> GHMERLLDELTLEGVARYMQSERCRRVICLVGAGISTSAGIPDFRSPSTGLYDNLEKYHLPYPEAIFEISYFKKHPEPFFALAKELYPGQFKPTICHYFMRLLKDKGLLLRCYTQNIDTLERIAGLEQEDLVEAHGTFYTSHCVSASCRHEYPLSWMKEKIFSEVTPKCEDCQSLVKPDIVFFGESLPARFFSCMQSDFLKVDLLLVMGTSLQVQPFASLISKAPLSTPRLLINKEKAGQSDPFLGMIMGLGGGMDFDSKKAYRDVAWLGECDQGCLALAELLGWKKELEDLVRREHASIDAQS;> EKR

NAD+-dependent protein deacylases (sirtuins) constitute a unique class of enzymes that are conserved from bacteria to humans. The human isotype Sirtuin 2 (Sirt2) deacetylates both nuclear and cytoplasmatic proteins and thereby functions as a major cell cycle regulator, a determinant of myelination, a regulator of autophagy and a suppressor of brain inflammation. In this work, we present the first crystal structures of Sirt2 in complex with a potent and Sirt2-selective small-molecule inhibitor with drug-like properties.

In the course of the investigation SirReal-mediated inhibition, we also determined the crystal structure of another aminothiazole, termed SirReal1 (2), in complex with Sirt2 and a different acetyl-lysine peptide substrate. The latter is derived from ornithine transcarbamoylase (OTC, structure termed Sirt2–SirReal1–OTC). SirReal1 has a benzyl instead of a naphthylmethyl substituent on the aminothiazole and is 26-fold less potent than SirReal2 in the same in vitro assay, but it retains high Sirt2 selectivity and shows similar behaviour in thermal stability assays. SirReal1 also locks Sirt2 in the open conformation and shows an almost identical interaction pattern as observed for SirReal2. In the Sirt2 complex with SirReal1, the acetyl-lysine-binding mode is different. The acetyl-lysine adopts an almost physiological position, as it is observed in the above-mentioned ternary sirtuin complexes. However, even in case of SirReal1, the benzyl moiety of SirReal1 shifts the acetyl-lysine of the OTC peptide towards His187, weakening the formation of the hydrogen bond between the Nε–H of the acetyl-lysine and the backbone carbonyl-O of the conserved valine (distance between carbonyl-O of valine and Nε-KAc: 3.2 Å in Sirt2–SirReal1–OTC, 2.5–2.7 Å in ternary complexes). SirReal2 is partially non-competitive and SirReal1 is competitive towards NAD+. Both SirReal inhibitors also exhibit acetyl-lysine competition with inhibition constants of 0.22 μM for SirReal2 and 3.33 μM for SirReal1.> 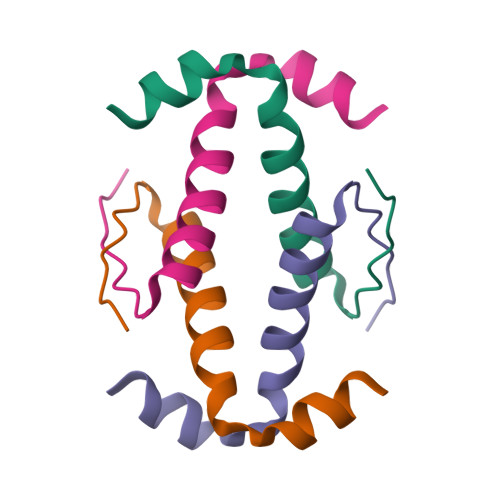GSDELLYLPVRGRETYEMLLKIKESLELMQYLPQHTIETYRQQQQQ> MAGQSTHYLAFPRASTITWGDDTRYWSWATVDFCSYAIE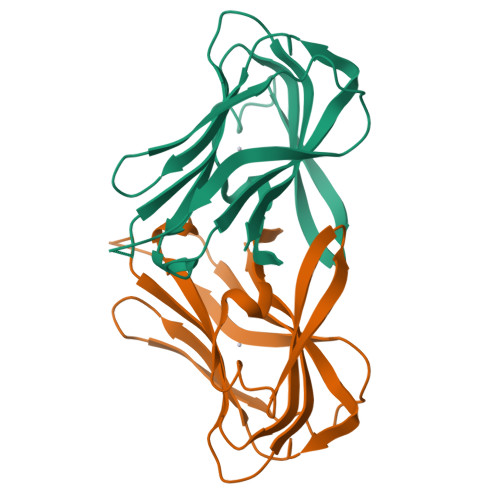EARLLQVSWLDCRWSMDASDFKQDIWYNASVEVMLTSNASGWNVPLHLEIELPDGSKQESQIVLAGRQPNVWFKIPIGKFILRGSLTSGTIRFGFYNHEGNWKRGLNIRTLAIQA> VVRVADTMPSGPSNSESIPALTAAETGHTSQVVPSDTIQTRHVRNFHVRSESSVENFLSRSACVYIVEYKTRDDTPDKMYDSWVINTRQVAQLRRKLEFFTYVRFDVEVTFVITSVQDDSTRQNTDTPALTHQIMYVPPGGPIPQAVDDYNWQTSTNPSVFWTEGNAPPRMSIPFMSVGNAYSNFYDGWSHFSQTGVYGFNTLNNMGKLYFRHVNDKTISPITSKVRIYFKPKHVKAWVPRPPRLCEYTHKDNVDFEPKGVTTSRTQLTISNS;> SDRVRSITLGNSTITTQESANVVVGYGVWPDYLSDEEATAEDQPTQPDVATCRFYTLDSVSWMKESQGWWWKFPDALRDMGLFGQNMQYHYLGRSGYTIHVQCNASKFHQGCLLVVCVPEAEMGAANINEKINREHLSNGEVANTFSGTKSSNTNDVQQAVFNAGMGVAVGNLTIFPHQWINLRTNNCATIVMPYINSVPMDNMFRHY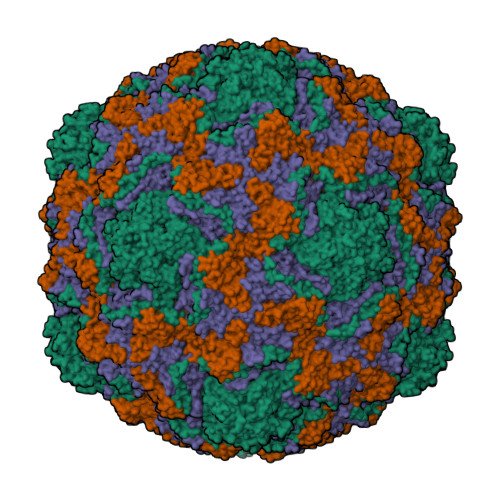NFTLMIIPFAKLDYAAGSSTYIPITVTVAPMCAEYNGLRLAGHQ;> GLPVMNTPGSNQFLTSDDYQSPTAMPQFDVTPEMNIPGEVKNLMEIAEVDSVVPVNNVNENVNSLEAYRIPVHSVTETGAQVFGFTLQPGADTVMERTLLGEILNYYANWSGSIKLTFMYCGSAMATGKFLLAYSPPGAGVPKNRREAMLGTHIIWDIGLQSSCVLCVPWISQTHYRFVSKDIYTDAGFITCWYQTSIVVPAEVQNQSVILCFVSACNDFSVRLLRDSPFVRQTAFYQ;> GAQVSTQKTGAHETSLSASGNSTIHYTNINYYKDAASNSANRQDFTQDPGKFTEPVKDIMVKSLPALN> MSEEEVSFSRDYFVEMDVRDEEAHELASDWFDEVVFTKKLVLEDPPDWGSLKEELKELRGKYGKVALLLVTRKPSLIREVKSRNLKALLYVQGGDMRINRMAIESGVDALI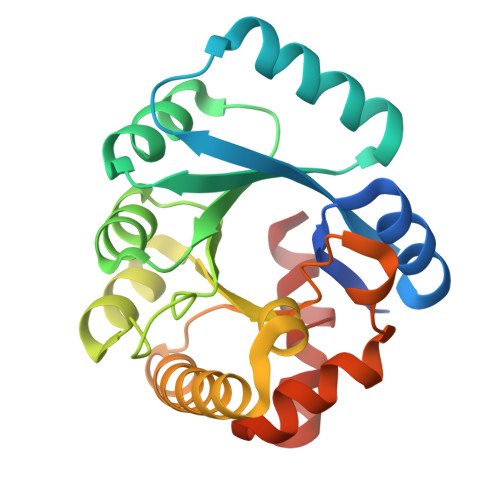SPWFGRKDPGFDHTLAGMAARRGVAIGFSLSPLLNANPYGRAQILRFMMKTWQLVKKYRVPRFITSSAESRWEVRGPRDLMSLGINIGMEIPEARASLNFYPRTIVWKL>[8x]MATTSNQNVEFVRTGYGKNMVKVLHIRREGNHHHIIELIANVQLTLKTRKDYLTGDNSDIIPTDTVKNTVHALAKLKGIKSIESFALDICEHF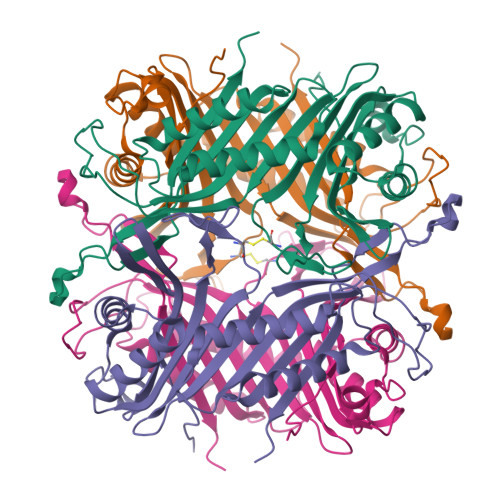LTAFNHVTRVKVNIDEVPWKRLEKNGVEHNHAFIHCPEALRFCEAEQYLSKTPVVHSGLKDMKVLKTTQTGFEGFLRDRFTTLTDAKDRFFCTSVYARWRYNTINVAFDAAWKAVKDTVIQKFAGPYDRGEYSPSVQKTLYDTQLLVLDRIPEVEEIEIIMPNQHYFVIDMTKIGLSNKDEVYLPLDNPSGNITGTVCRKPRARM> NVEEETKYIELMIVNDHLMFKKHRLSVVHTNTYAKSVVNMADLIYKDQLKTRIVLVAMETWATDNKFAISENPLITLREFMKYRRDFIKEKSDAVHLFSGSQFESSRSGAAYIGGICSLLKGGGVNEFGKTDLMAVTLAQSLAHNIGIISDKRKLASGECKCEDTWSGCIMGDTGYYLPKKFTQCNIEEYHDFLNSGGGACLFNKPSKLLDPPECGNGFIETGEECDCGTPAECVLEGAECCKKCTLTQDSQCSDGLCCKKCKFQPMGTVCREAVNDCDIRETCSGNSSQCAPNIHKMDGYSCDGVQGICFGGRCKTRDRQCKYIWGQKVTASDKYCYEKLNIEGTEKGNCGKDKDTWIQCNKRDVLCGYLLCTNIGNIPRLGELDGEITSTLVVQQGRTLNCSGGHVKLEEDVDLGYVEDGTPCGPQMMCLEHRCLPVASFNFSTCLSSKEGTICSGNGVCSNELKCVCNRHWIGSDCNTYFPHN;>DAAQPARRARRTYEAYPAKPKCPAVCTCTKDNALCENARSIPRTVPPDVISLSFVRSGFTEISEGSFLFTPSLQLLLFTSNSFDVISDDAFIGLPHLEYLFIENNNIKSISRHTFRGLKSLIHLSLANNNLQTLPKDIFKGLDSLTNVDLRGNSFNCDCKLKWLVEWLGHTNATVEDIYCEGPPEYKKRKINSLSSKDFDCIITEFAKSQDLPYQSLSIDTFSYLNDEYVVIAQPFTGKCIFLEWDHVEKTFRNYDNITGTSTVVCKPIVIETQLYVIVAQLFGGSHIYKRDSFANKFIKIQDIEILKIRKPNDIETFKIENNWYFVVADSSKAGFTTIYKWNGNGFYSHQSLHAWYRDTDVEYLEIVRTPQTLRTPHLILSSSSQRPVIYQWNKATQLFTNQTDIPNMEDVYAVKHFSVKGDVYICLTRFIGDSKVMKWGGSSFQDIQAMPSRGSMVFQPLQINNYQYAILGSDYSFTQVYNWDAEKAKFVKFQELNVQAPRSFTHVSINKRNFLFASSFKGNTQIYKHVIVDLSAKHHHHHH[2x]

LGI1 is a 60 kDa secreted neuronal protein that consists of the N-terminal leucine-rich repeat (LRR) domain and the C-terminal epitempin-repeat (EPTP) domain (Staub et al., 2002). Meanwhile, the S473L mutation of LGI1 causes epileptiform seizures due to reduced binding to ADAM22, which is a member of the A disintegrin and metalloproteinase (ADAM) family and acts as a receptor for LGI1 in neurons without protease activity. The ectodomain (ECD) of ADAM22 consists of a metalloprotease-like domain, a disintegrin domain, a cysteine-rich domain, and an EGF-like domain (Liu et al., 2009). As such, the LGI1–ADAM22 complex maintains normal nerve signal transduction through the interaction network, including synaptic ion channels.

We also determined the 3D structure of the LGI1LRR–LGI1EPTP–ADAM22ECD complex at a nominal resolution of 2.78 Å. Nonuniform refinement using the particle images with the original pixel size yielded a density map at a nominal resolution of 2.78 Å. This map corresponds to a part of the 3:3 complex, where two-thirds of the complex may adopt various conformations. In the cryo-EM structure of the LGI1LRR–LGI1*EPTP–ADAM22ECD complex, the LGI1EPTP–ADAM22ECD structure is essentially identical to that determined by X-ray crystallography. At the interface, Trp398, Tyr408, and Tyr409 of ADAM22 are stacked in a layer and project into the hydrophobic inner rim of the central channel of LGI1EPTP, which consists of Leu237, Phe256, Val284, Leu302, Tyr433, Met477, and Phe541 of LGI1. In addition, several hydrogen bonds are formed between LGI1 and ADAM22: Arg330 and Lys353 of LGI1 form hydrogen bonds with Asp405 and Glu359 of ADAM22, respectively, whereas Arg378 of LGI1 forms hydrogen bonds with Ser340 and Thr406 of ADAM22. The hydrogen bond between Asp431 of LGI1 and Lys362 of ADAM22 was also found in the cryo-EM structure. Specifically, Glu123 and Arg76 of LGI1LRR form hydrogen bonds with Arg474 and Glu516 of LGI1*EPTP, respectively. The hydrogen bond between Glu123 of LGI1LRR and Arg474 of LGI*EPTP is reinforced by stacking with Phe121 of LGI1LRR. The present higher-resolution structure demonstrates that Arg474 of LGI1*EPTP forms a hydrogen bond with Glu123 of LGI1LRR, which was ambiguous in the previous moderate-resolution crystal structure. No tight interaction was found between LGI1LRR and ADAM22ECD in the cryo-EM structure of the LGI1LRR–LGI1*EPTP–ADAM22ECD complex.>[2x]MRKYAAIALCTSAILAGCNTSNVSQE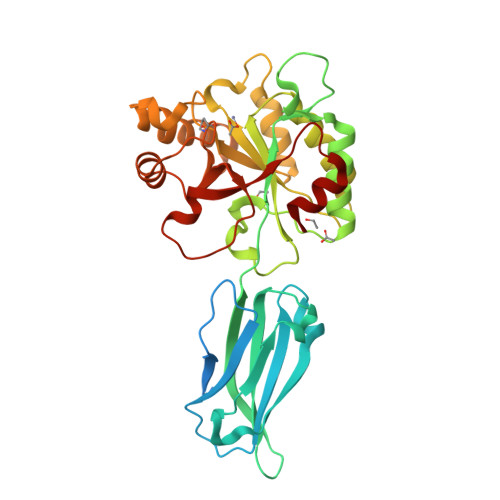PNKERKVQETKKQAETVQEQGKISYNPITHESTNTTIHMTDIKDTLTEVQYKIWRTADGKETAKSLSSKEKEKQFSLPFDTKEFEGKRGEFQIEAIGIKEDGKTIPLTKSAITFEQKVPVLMYHAIDDYHGQGIKDLFVSPANFEAQMKYLKDNGYTLLTFERWGDINKVNKPIFVTFDDGMKNNMNAFHVLQKLKDDTFKPVATEYMIVNNVDAEGSLSTSDIKEMVDSGIFSMQSHTATHADLPKITNYEEELKESKEKLEKITGKPVIAVAYXFGHVDDKVVAETKKYYQFATTTKPGKFITKGEPDELLKMKRVRIHHTTTVEQFASSIK>[2x]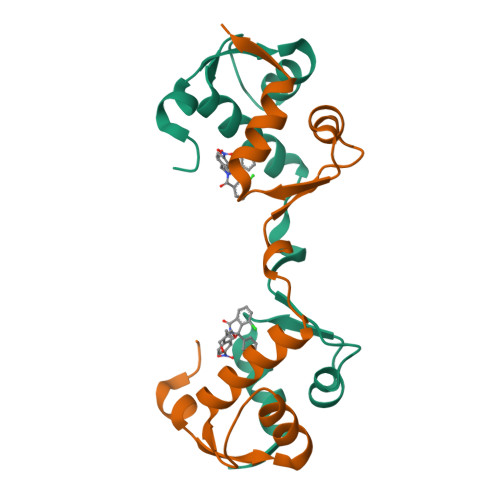GPLGSSQIPASEQETLVRPKPLLLKLLKSVGAQKDTYTMAEVLFYLGQYIMTKRLYDEKQQHIVYCSNDLLGDLFGVPSFSVKEHRKIYTMIYRNLVVVNQQESSDSGTSVSEN Norrie Disease Protein (NDP) gene encodes Norrin, a secreted cystine-knot like growth factor, distinct from the lipid-modified Wnt. Unlike Wnts which have promiscuous interactions with Fz receptors, Norrin specifically binds to Fz4CRD, but not to the 14 other CRDs of Fz and secreted Frizzled-related protein (sFRP) family members. The Norrin mediated pathway maintains the blood-retina and blood-brain barriers and regulates angiogenesis in the cochlea and uterus as well as neuroprotective effects on retinal neurons. Our crystallographic and solution studies further reveal that dimeric Norrin forms a complex with two copies of monomeric Fz4CRD.

We purified Norrin–Fz4CRD complex and determined the crystal structures of methylated Norrin–Fz4CRD (dimethylated surface-exposed lysine residues) and Norrin–Fz4CRD–SOS (complex bound with heparin mimic sucrose octasulfate, SOS) at 2.3 Å and 3.0 Å resolution, respectively. These two complex structures show different stoichiometries: a 2:1 complex for the methylated Norrin–Fz4CRD and a 2:2:2 stoichiometry for the Norrin–Fz4CRD–SOS complex, the architecture of which resembles a butterfly. Thus although the methylated Norrin–Fz4CRD structure usefully provides high-resolution information for the ligand–receptor interface, the Norrin–Fz4CRD–SOS structure defines the overall architecture of the native complex. The Norrin–Fz4CRD binding interface is conserved between the complex structures. Each Fz4CRD interacts one-to-one with a separate Norrin chain, burying on average 1680 Å2 of surface area. At the ligand–receptor interface two β-hairpins in Norrin (β1-β2 and β5-β6) contact three loops in Fz4CRD (I, II, and III). Interactions with SOS involve the positively charged residues of Lys58, Arg107, Arg109, and Arg115 on Norrin, plus His154 and Asn155 on Fz4CRD loop III. We have discovered a GAG binding site that may span Norrin and Fz4CRD. We propose that the extended GAG binding site may allow co-receptor HSPGs to recruit secreted Norrin for interaction with Fz4CRD and to co-localize Norrin and Fz4 receptor, similar to the role of HSPGs in Wnt signalling. Secondly, we show the Norrin dimer binds separately to two molecules of Fz4CRD, in contrast to the 1:1 complex of Wnt8–Fz8CRD.

> GPGKTDSSFIMDSDPRRCMRHHYVDSISHPLYKCSSKMVLLARCEGHCSQASRSEPLVSFSTVLKQPFRSSCHCCRPQTSKLKALRLRCSGGMRLTATYRYILSCHCEECNSGTETSQVAPA;> DTGERRCDPIRISMCQNLGYNVTKMPNLVGHELQTDAELQLTTFTPLIQYGCSSQLQFFLCSVYVPMCTEKINIPIGPCGGMCLSVKRRCEPVLKEFGFAWPESLNCSKFPPQNDHNHMCMEGPGDEEVPLPHKTPIQPGEGTLEVLFQ> GSHMSPLLQPGLAALRRRAREAGVPLAPLPLTDSFLLRFLRARDFDLDLAWRLLKNYYKWRAECPEISADLHPRSIIGLLKAGYHGVLRSRDPTGSKVLIYRIAHWDPKVFTAYDVFRVSLITSELIVQEVETQRNGIKAIFDLEGWQFSHAFQITPSVAKKIAAVLTDSFPLKVRGIHLINEPVIFHAVF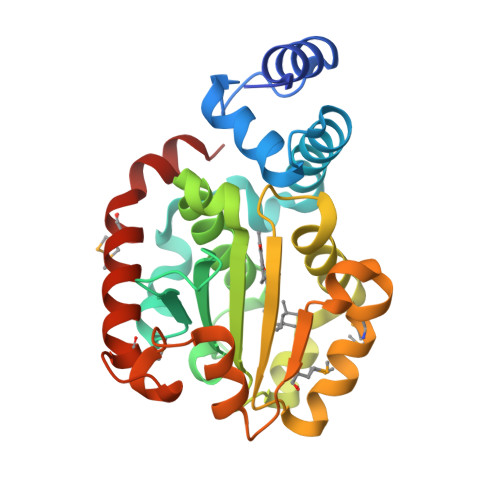SMIKPFLTEKIKERIHMHGNNYKQSLLQHFPDILPLEYGGEEFSMEDICQEWTNFIMKSEDYLSSISESIQ> GTSSMADIG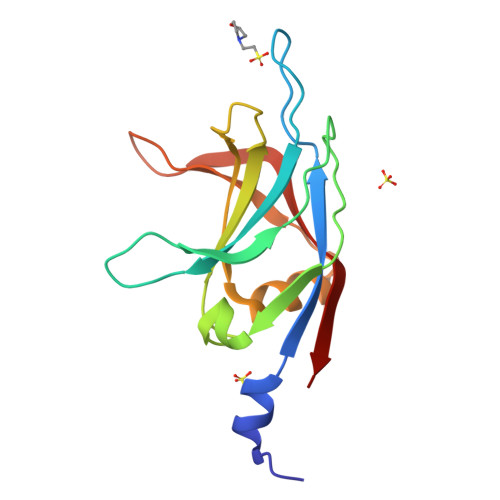SKISTEIVFRCSNLESKDLFSKSDPFLVVSKIVEHGTPIPVSKTEVRKNDLNPIWKPVFLSVQQVGSKDSPVIIECSDFNSNGKHSLIGKVQKSLSDLEKLHLAGQGINFSLPTGAGQNKVLKSQLFVDKFTETV> MWQAFKNAFKIPELRDRIIFTFLALIVFRMGIYIPVPGLNLEAWGEIFRRIAETAGVAGILSFYDVFTGGALSRFSVFTMSVTPYITASIILQLLASVMPSLKEMLREGEEGRKKFAKYTRRLTLLIGGFQAFFVSFSLARSNPDMVAPGVNVLQFTVLSTMSMLAGTM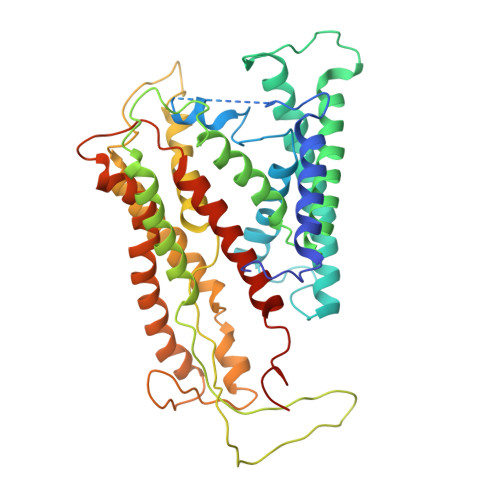FLLWLGERITEKGIGNGISILIFAGIVARYPSYIRQAYLGGLNLLEWIFLIAVALITIFGIILVQQAERRITIQYARRVTGRRVYGGASTYLPIKVNQGGVIPIIFASAIVSIPSAIASITNNETLKNLFRAGGFLYLLIYGLLVFFFTYFYSVVIFDPREISENIRKYGGYIPGLRPGRSTEQYLHRVLNRVTFIGAVFLVVIALLPYLVQGAIKVNVWIGGTSALIAVGVALDIIQQMETHMVMRHYEGFIKKGKIRGRR>[4x]GSGSHVTLPFYPKSPQSKDLIKEAILDNDFMKNLELSQIQEIVDCMYPVEYGKDSCIIKEGDVGSLVYVMEDGKVEVTKEGVKLCTMGPGKVFGELAILYNCTRTATVKTLVNVKLWAIDRQCFQTIMMRTGLIKHTEY

The cGMP-dependent protein kinases (PKG) belong to the family of serine/threonine kinases and are one of the major intracellular receptors for cGMP. Next, two cyclic-nucleotide binding domains (CNBD-A and CNBD-B) are followed by the catalytic domain. Binding of cGMP to the CNBDs is thought to induce a conformational change that activates the kinase by removing the autoinhibitory domain from the catalytic cleft, leaving the catalytic domain free to phosphorylate downstream substrates. To understand the overall architecture of the cGMP-binding domain and the molecular features required for cGMP binding, we determined crystal structures of the CNBD-A of human PKG I bound to cGMP, cAMP or in the absence of bound nucleotide.

Our attempts to obtain crystal structures of an apo form of the CNBD-A yielded a partial apo structure, where two of the four molecules in the unit cell were bound by cAMP (CNBD-A:cAMPP43), which came from the E. coli cultures. Molecules without cAMP were bound by phosphate (CNBD-A:PO4), possibly due to high concentration of phosphate in the crystallizing solution. CNBD-A:PO4 superimposes well with CNBD-A:cAMPP43, except for the β4 and β5 strands. In the absence of cAMP, this region moves slightly away from the PBC resulting in a more open conformation. In contrast to our CNBD-A:cAMP complex, where a full electron density was seen for cAMP bound in two different configurations, only partial electron density was seen for each bound cAMP in two of the four molecules in the CNBD-A:cAMPP43 crystal, which accounts only for the sugar phosphate moiety and pyrimidine portion of the adenine ring. This partial density can be explained by either syn- or anti-configured cAMP indiscriminately binding to the cGMP pocket, since either configuration of cAMP can be fitted to the partial electron density. The phosphate molecule, binds the same site as the cyclic phosphates, with the same set of interactions. The partial-apo structure was crystallized in a P43 space group and contained four molecules per unit cell, showing a set of crystal contacts that are different from the PKG Iβ:cAMP and PKG Iβ:cGMP complexes. In the absence of cyclic nucleotides, the conformation of CNBD-A is similar to the cyclic-nucleotide bound forms; with the exception of the β4/β5 strands which are in an open conformation with respect to PBC, as seen in the PO4 bound structure. PKG Iβ:cGMP and partial-apo structures were subsequently solved at 2.9 Å and 2.75 Å respectively, using the fully refined structure of the PKG Iβ:cAMP complex as a molecular replacement model.> TQVAKKILVTCALPYANGSIHLGHMLEHIQADVWVRYQRMRGHEVNFICADDAHGTPIMLKAQQLGITPEQMIGEMSQEHQTDFAGFNISYDNYHSTHSEENRQLSELIYSRLKENGFIKNRTISQLYDPEKGMFLPDRFVKGTCPKCKSPDQYGDNCEVCGATYSPTELIEPKSVVSGATPVMRDSEHFFFDLPSFSEMLQAWTRSGALQEQVANKMQEWFESGLQQWDISRDAPYFGFEIPNAPGKYFYVWLDAPIGYMGSFKNLCDKRGDSVSFDEYWKKDSTAELYHFIGKDIVYFHSLFWPAMLEGSNFRKPSNLFVHGYVTVNGAKMSKSRGTFIKASTWLNHFDADSLRYYYTAKLSS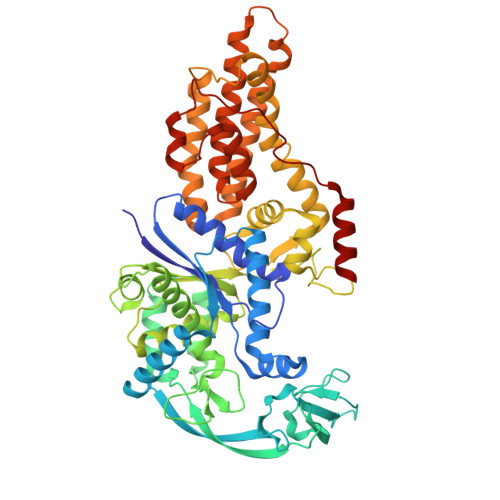RIDDIDLNLEDFVQRVNADIVNKVVNLASRNAGFINKRFDGVLASELADPALYKTFTDAAEVIGEAWESREFGKAVREIMALADLANRYVDEQAPWVVAKQAGRDADLQAICSMGINLFRVLMTYLKPVLPKLTERAEAFLNTELTWDGIQQPLLGHKVNPFKALYNRIDMRQVEALVEASKEEVK>[2x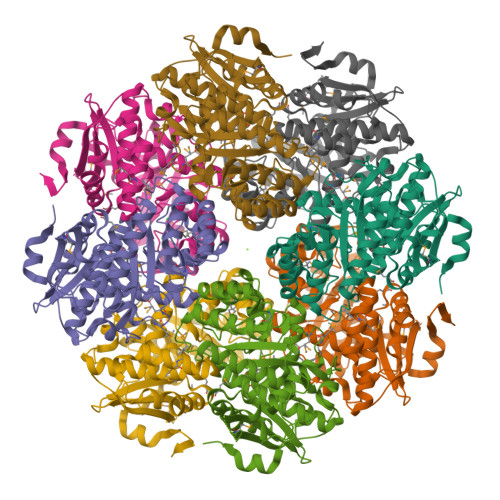]MSLKIAKVEALSVAMGDGTGWMPTSAFVRITAEDGTVGWGEASPMLGGIASLGVVARDIAPFLEGQEVLDHAVLLDRMMHRLVKLGPEGIATAALAACDIALWDLKGKLLGQPIYKLLGGAWRTRLPCYSSIGGNAARSVDEVVREVARRVEAEQPAAVKIRWDGDRTRCDVDIPGDIAKARAVRELLGPDAVIGFDANNGYSVGGAIRVGRALEDLGYSWFEEPVQHYHVGAMGEVAQRLDITVSAGEQTYTLQALKDLILSGVRMVQPDIVKMGGITGMMQCAALAHAHGVEFVPHQTQPGVGHFANIHVLSTLMHMTKPVELADRWDRGRPVFRNPAEPVDGHFALGDAPGLGIVVDEDELASRATEITVGRDQRPPAGGQYEGHHHHHH>MMPIKSIVTLDQLEDSEYLFRIVSTVLPHLCLDYKVCDQLKTTFVHPFDILLNNSLGSVTKQDELQAAISKLGINYLIDTTSRELKLFNVTLNAGNIDIINTPINISSETNPIINTHSFYDLPPFTQHLLNIRLTDTEYRARFIGGYIKPDGSDSMDVLAEKKYPDLNFDNTYLFNILYKDVINAPIKEFKAKIVNGVLSRQDFDNLIGVRQYITIQDRPRFDDAYNIADAARHYGVNLNTLPLPNVDLTTMPTYKHLIMFEQYFIYTYDRVDIYYNGNKMLFDDEIINFTISMRYQSLIPRLVDFFPDIPVNNNIVLHTRDPQNAAVNVTVALPNVQFVDINRNNKFFINFFNLLAKEQRSTAIKVTKSMFWDGMDYEEYKSKNLQDMMFINSTCYVFGLYNHNNTTYCSILSDIISAEKTPIRVCLLPRVVGGKTVTNLISETLKSISSMTIREFPRKDKSIMHIGLSETGFMRFFQLLRLMADKPHETAIKEVVMAYVGIKLGDKGSPYYIRKESYQDFIYLLFASMGFKVTTRRSIMGSNNISIISIRPRVTKQYIVATLMKTSCSKNEAEKLITSAFDLLNFMVSVSDFRDYQSYRQYRNYCPRYFYAG[3x];>[3x]MDFFNKFSQGLAESSTPKSSIYYSEEKDPDTKKDEAIEIGLKSQESYYQRQLREQLARDNMTVASRQPIQPLQPTIHITPQPVPTATPAPILLPSSTVPTPKPRQQTNTSSDMSNLFDWLSEDTDAPASSLLPALTPSNAVQDIISKFNKDQKTTTPPSTQ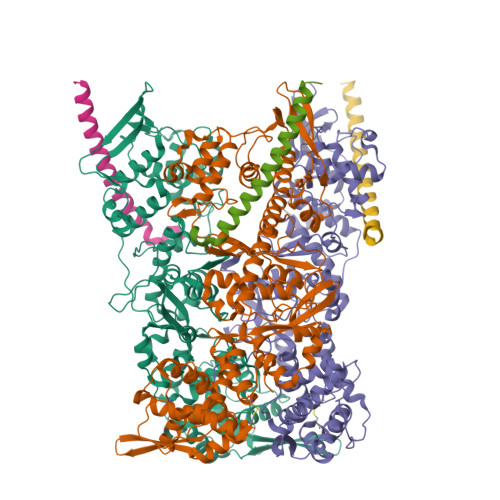PSQTLPTTTCTQQSDGNISCTTPTVTPPQPPIVATVCTPTPTGGTVCTTAQQNPNPGAASQQNLDDMALKDLMSNVERDMHQLQAETNDLVTNVYDAREYTRRAIDQILQLVKGFERFQK>[2x]GQFTGTGTGGDVFKVDLNEQFDRADMVWIGTASVLVWIMIPGVGLLYSGISRKKHALSLMW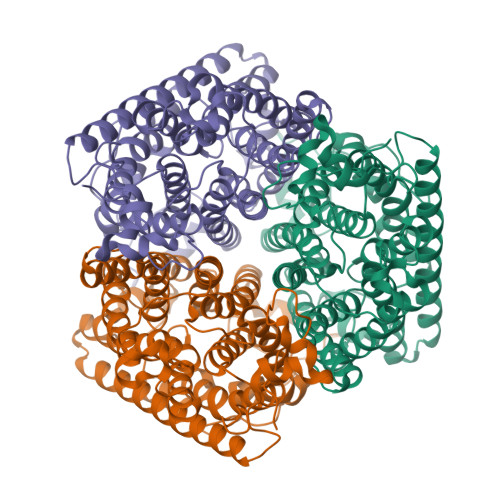AALMAACVAAFQWFWWGYSLVFAHNGSVFLGTLQNFCLKDVLGAPSIVKTVPDILFCLYQGMFAAVTAILMAGAGCERARLGPMMVFLFIWLTVVYCPIAYWTWGGNGWLVSLGALDFAGGGPVHENSGFAALAYSLWLGKRHDPVAKGKVPKYKPHSVSSIVMGTIFLWFGWYGFNGGSTGNSSMRSWYACVNTNLAAATGGLTWMLVDWFRTGGKWSTVGLCMGAIAGLVGITPAAGYVPVYTSVIFGIVPAIICNFAVDLKDLLQIDDGMDVWALHGVGGFVGNFMTGLFAADYVAMIDGTEIDGGWMNHHWKQLGYQLAGSCAVAAWSFTVTSIILLAMDRIPFLRIRLHEDEEMLGTDLAQIGEYAYYADDDPETNPYVLEPIRS> PELPEVETVRRELEKRIVGQKIISIEATYPRMVLTGFEQLKKELTGKTIQGISRRGKYLIFEIGDDFRLISHLRMEGKYRLAT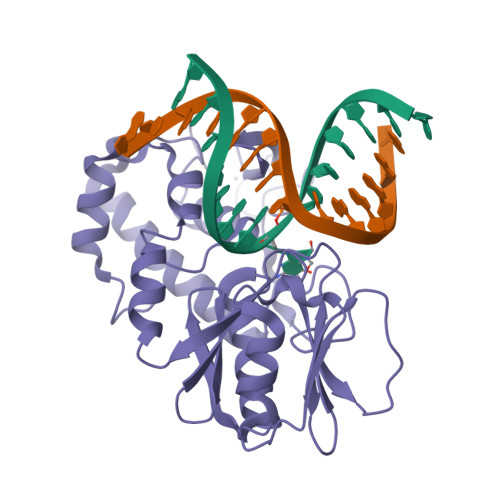LDAPREKHDHLTMKFADGQLIYADVRKFGTWELISTDQVLPYFLKKKIGPEPTYEDFDEKLFREKLRKSTKKIKPYLLEQTLVAGLGNIYVDEVLWLAKIHPEKETNQLIESSIHLLHDSIIEILQKAIKLGGSSIRPYSALGSTGKMQNELQVYGKTGEKCSRCGAEIQKIKVAGRGTHFCPVCQQK> ENSEVIKDLYEYLCNVRVHKSYEDDSGLWFDISQGTHSGGSSDDYSIMDYKLGFVKGQAQVTEV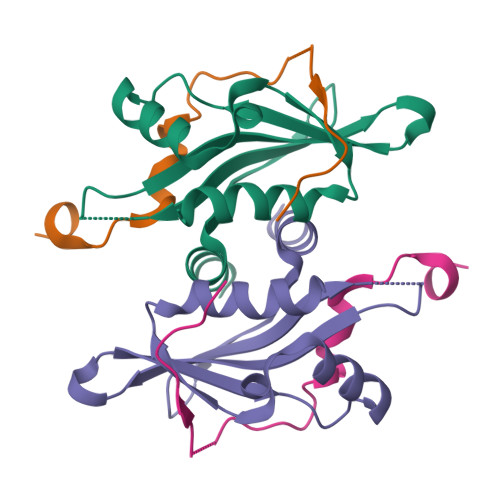IYAPVLKQRSTEELYSLQSKLPEYLFETLSFPLSSLNQFYNKIAKSLNK;> SNAPYFGRPSLKTRAKQFEGVSSKDIGENCRRIEAFSD> MKIRAKVELTWEY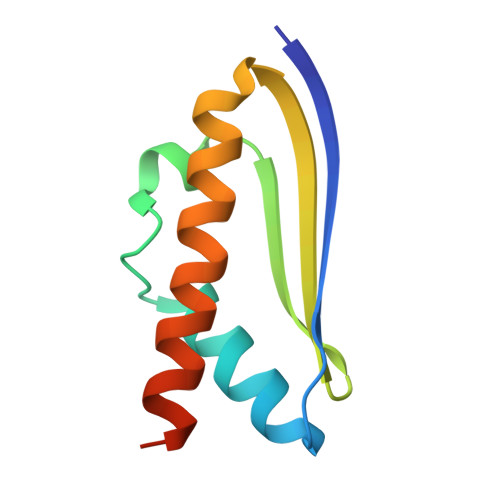EDEETAKAIANAVNVDNISIPEKLKKSLNLITFPDGARVVTKVKYEGEIESLVVALDDLIFAIKVAEEVLWSHPQFEK1-HEPTADECANOYL-2-TRIDECANOYL-3-GLYCEROL-PHOSPHONYL CHOLINE | C38 H77 N O8 P 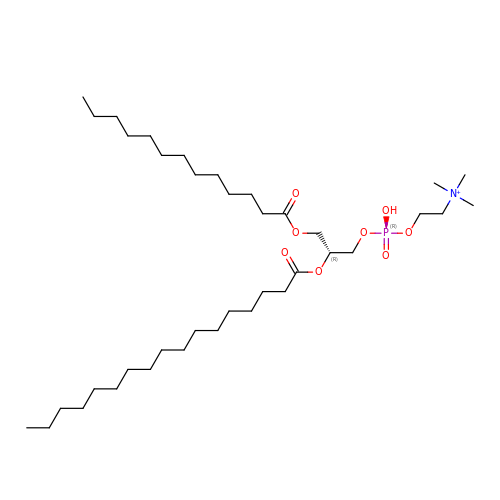| AZEAMUNCULVBPK-PSXMRANNSA-O> LPTPASLNGNTEVATISDVKLEARSDTTYHKCSKC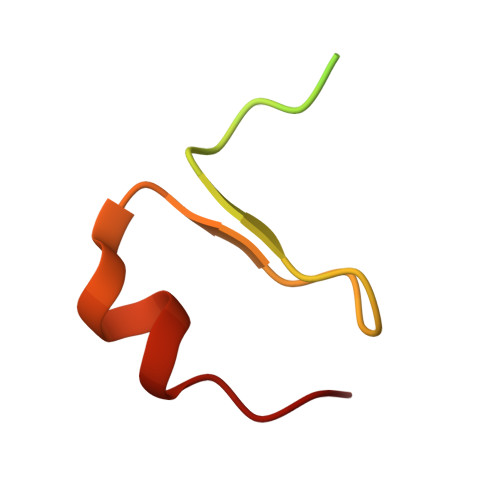GYGSDDSDAYFNHKCN> MERTELLKPRTLADLIRILHELFAGDEVNVEEVQAVLEAYESNPAEWALYAKFDQYRYTRNLVDQGNGKFNLMILCWGEGHGSSIHDHTDSHGFLKLLQGNLKETLFDWPDKKSNEMIKKSERTLRENQCAYINDSIGLHRVENVSHTEPAVSLHLYSPPFDTCHAFDQRTGHKNKVTMTFH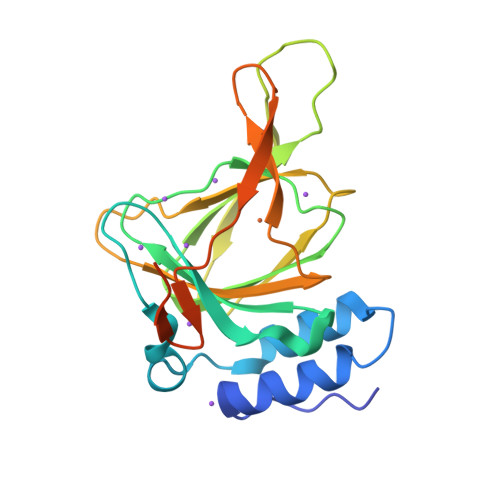SKFGIRTPFTTSGSLENNSAWSHPQFEK> MSLYRRLVLLSCLSWPLAGFSATALTNLVAEPFAKLEQDFGGSIGVYAMDTGSGATVSYRAEERFPLCSSFKGFLAAAVLARSQQQAGLLDTPIRYGKNALVPWSPISEKYLTTGMTVAELSAAAVQYSDNAAANLLLKELGGPAGLTAFMRSIGDTTFRLDRWELELASAIPGDARDTSSPRAVTESLQKLTLGSALAAPQRQQFVDWLKGNTTGNHRIRAAVPADWAVGDKTGTCGVYGTANDYAVVWPTGRAPIVLAVYTR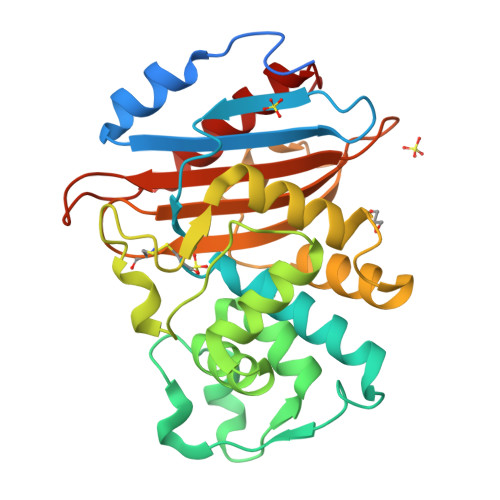APNKDDKHSEAVIAAAARLALEGLGVNGQ> PVTINNFNYNDPIDNNNIIMMEPPFARGTGRYYKAFKITDRIWIIPERYTFGYKPEDFNKSSGIFNRDVCEYYDPDYLNTNDKKNIFLQTMIKLFNRIKSKPLGEKLLEMIINGIPYLGDRRVPLEEFNTNIASVTVNKLISNPGEVERKKGIFANLIIFGPGPVLNENETIDIGIQNHFASREGFGGIMQMKFCPEYVSVFNNVQENKGASIFNRRGYFSDPALILMHELIHVLHGLYGIKVDDLPIVPNEKKFFMQSTDAIQAEELYTFGGQDPSIITPSTDKSIYDKVLQNFRGIVDRLNKVLVCISDPNININIYKNKFKDKYKFVEDSEGKYSIDVESFDKLYKSLMFGFTETNIAENYKIKTRASYFSDSLPPVKIKNLLDNEIYTIEEGFNISDKDMEKEYRGQNKAINKQAYEEISKEHLAVYKIQMCKSVKAPGICIDVDNEDLFFIADKNSFSDDLSKNERIEYNTQSNYIENDFPINELILDTDLISKIELPSENTESLTDFNVD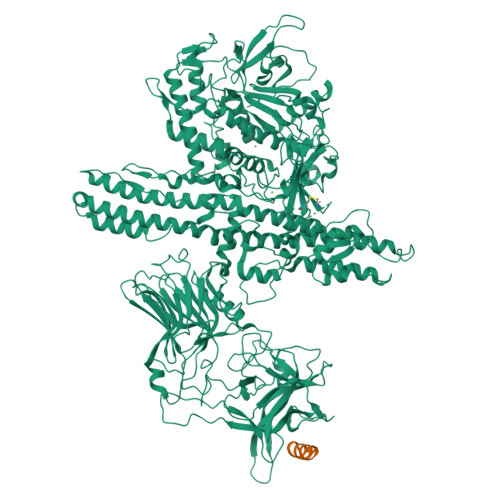VPVYEKQPAIKKIFTDENTIFQYLYSQTFPLDIRDISLTSSFDDALLFSNKVYSFFSMDYIKTANKVVEAGLFAGWVKQIVNDFVIEANKSNTMDKIADISLIVPYIGLALNVGNETAKGNFENAFEIAGASILLEFIPELLIPVVGAFLLESYIDNKNKIIKTIDNALTKRNEKWSDMYGLIVAQWLSTVNTQFYTIKEGMYKALNYQAQALEEIIKYRYNIYSEKEKSNINIDFNDINSKLNEGINQAIDNINNFINGCSVSYLMKKMIPLAVEKLLDFDNTLKKNLLNYIDENKLYLIGSAEYEKSKVNKYLKTIMPFDLSIYTNDTILIEMFNKYNSEILNNIILNLRYKDNNLIDLSGYGAKVEVYDGVELNDKNQFKLTSSANSKIRVTQNQNIIFNSVFLDFSVSFWIRIPKYKNDGIQNYIHNEYTIINCMKNNSGWKISIRGNRIIWTLIDINGKTKSVFFEYNIREDISEYINRWFFVTITNNLNNAKIYINGKLESNTDIKDIREVIANGEIIFKLDGDIDRTQFIWMKYFSIFNTELSQSNIEERYKIQSYSEYLKDFWGNPLMYNKEYYMFNAGNKNSYIKLKKDSPVGEILTRSKYNQNSKYINYRDLYIGEKFIIRRKSNSQSINDDIVRKEDYIYLDFFNLNQEWRVYTYKYFKKEEEKLFLAPISDSDEFYNTIQIKEYDEQPTYSCQLLFKKDEESTDEIGLIGIHRFYESGIVFEEYKDYFCISKWYLKEVKRKPYNLKLGCNWQFIPKDEGWTE;> GESQEDMFAKLKEKFFNEINK>GPLGSETITVPTPIKQIFSDDAFAETIKDNLKKKSVTDAVTQNELNSIDQIIANNSDIKSVQGIQYLPNVTKLFLNGNKLTDIKPLANLKNLGWLFLDENKVKDLSSLKDLKKLKSLSLEHNGISDINGLVHLPQLESLYLGNNKITDITVLSRLTKLDTLSLEDNQISDIVPLAGLTKLQNLYLSKNHISDLRALAGLKNLDVLELFSQECLNKPINHQSNLVVPNTVKNTDGSLVTPEIISDDGDYEKPNVKWHLPEFTNEVSFIF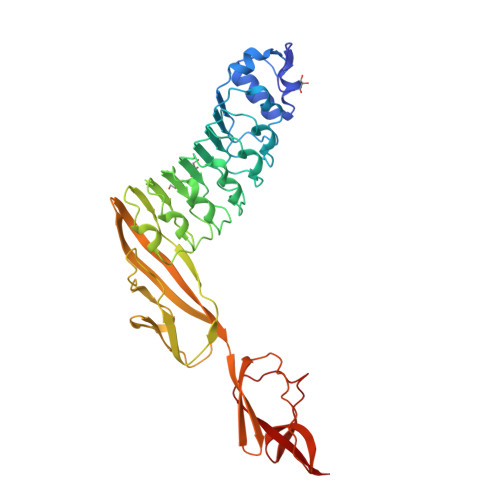YQPVTIGKAKARFHGRVTQPLKEVYTVSYDVDGTVIKYKVEAGTRITAPKPPTKQGYVFKGWYTEKNGGHEWNFNTDYMSGNDFTLYAVFKAET[3x]>GHMKKQLIEFVRWSPERAQHYRNKGYWIDQPLTRILTVGVQSHPHSLAIICGERQLSYIELDRLSTNLATRLAEKGLGKGDTALVQLPNVAEFYIVFFALLKAGVVVLNALYSHRQYELNAFIKQIQPKLLIGSRQHEVFSNNQFIDSLHDVNLSPEIILMLNHQATDFGLLDWIETPAETFVDFSSTPADEVAFFQLSGGSTGTPKLIPRTHNDYDYSVRASAEICGLNSNTRLLCALPAPHNFMLSSPGALGVLHAGGCVVMAPNPEPLNCFSIIQRHQVNMASLVPSAVIMWLEKAAQYKDQIQSLKLLQVGGASFPESLARQVPEVLNCKLQQVFGMAEGLVNYTRLDDSDEQIFTTQGRPISSDDEIKIVDEQYREVPEGEIGMLATRGPYTFCGYYQSPEHNSQVFDEDNYYYSGDLVQRTPDGNLRVVGRIKDQINRGGEKIASEEIEKLILLHPEVMHAALVAIVDEQFGEKSCAFIVSRNPELKAV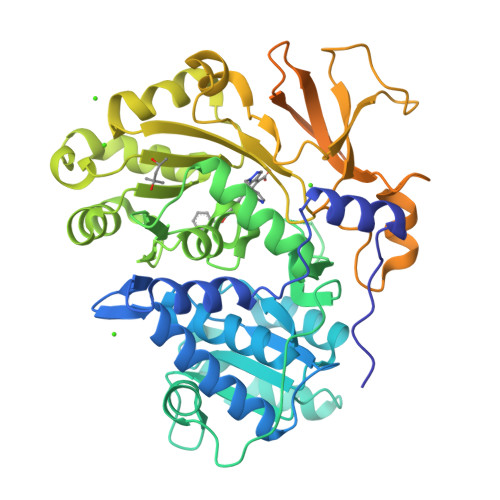VLRRHLMELGIAQYKLPDQIKLIESLPLTAVGKVDKKQLRSILNTSTTS[2x]>[4x]MSTPKIIYTLTDEAPALATYSLLPIIKAFTGSSGIAVETRDISLAGRLIATFPEYLTDTQKISDDLAELGKLATTPDANIIKLPNISASVPQLKAAIKELQQQGYKLPDYPEEPKTDTEKDVKARYDKIKGSAVNPVLREGNSDRRAPLSVKNYARKHPHKMGAWSADSKSHVAHMDNGDFYGSEKAALIGAPGSVKIELIAKDGSSTVLKAKTSVQAGEIIDSSVMSKNALRNFIAAEIEDAKKQGVLLSVHLKATMMKVSDPIMFGQIVSEFYKDALTKHAEVLKQIGFDVNNGIGDLYARIKTLPEAKQKEIEADIQAVYAQRPQLAMVNSDKGITNLHVPSDVIVDASMPAMIRDSGKMWGPDGKLHDTKAVIPDRCYAGVYQVVIEDCKQHGAFDPTTMGSVPNVGLMAQKAEEYGSHDKTFQIPADGVVRVTDESGKLLLEQSVEAGDIWRMCQAKDAPIQDWVKLAVNRARATN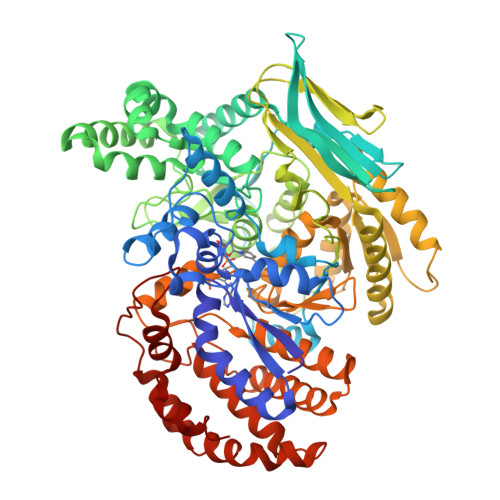TPAVFWLDPARAHDAQVIAKVERYLKDYDTSGLDIRILSPVEATRFSLARIREGKDTISVTGNVLRDYLTDLFPIMELGTSAKMLSIVPLMSGGGLFETGAGGSAPKHVQQFLEEGYLRWDSLGEFLALAASLEHLGNAYKNPKALVLASTLDQATGKILDNNKSPARKVGEIDNRGSHFYLALYWAQALAAQTEDKELQAQFTGIAKALTDNETKIVGELAAAQGKPVDIAGYYHPNTDLTSKAMRPSATFNAALAPLA>[10x]MAAQNEQRPERIKTTPYLEGDVLSSDSGPLLSVFALQEIMQKVRQVQADYMTATREVDFTVPDVQKILDDIKALAAEQVYKIVKVPSISFRHIVMQSRDRVLRVDTYYEEMSQVGDVITEDEPEKFYSTIIKKVRFIRGKGSFILHDIPTRDHRGMEVAEPEVLGVEFKNVLPVLTAEHRAMIQNALDGSIIENGNVATRDVDVFIGACSEPVYRIYNRLQGYIEAVQLQELRNSIGWLERLGHRKRITYSQEVLTDFRRQDTIWVLALQLPVNPQVVWDVPRSSIANLIMNIATCLPTGEYIAPNPRISSITLTQRITTTGPFAILTGSTPTAQQLNDVRKIYLALMFPGQIILDLKIDPGERMDPAVRMVAGVVGHLLFTAGGRFTNLTQNMARQLDIALNDYLLYMYNTRVQVNYGPTGEPLDFQIGRNQYDCNVFRADFATGTGYNGWATIDVEYREPAPYVHAQRYIRYCGIDSRELINPTTYGIGMTYHCYNEMLRMLVAAGKDSEAAYFRSMLPFHMVRFARINQIINEDLHSVFSLPDDMFNALLPDLIAGAHQNADPVVLDVSWISLWFAFNRSFEPTHRNEMLEVAPLIESVYASELSVMKVDMRHLSLMQRRFPDVLIQARPSHFWKAVLNDSPEAVKAVMNLSHSHNFINIRDMMRWVMLPSLQPSLKLALEEEAWAAANDFEDLMLTDQVYMHRDMLPEPRLDDIERFRQEGFYYTNMLEAPPEIDRVVQYTYEIARLQANMGQFRAALRRIMDDDDWVRFGGVLRTVRVKFYDARPPDDVLQGLPFSYDTNERGGLAYATIKYATETTIFYLIYNVEFSNTPDSLVLINPTYTMTKVFINKRIVERVRVGQILAVLNRRFVAYKGKMRIMDITQSLKMGTKLAAPTV;> MVAITVQGAQLIKRVVERFYPGIAFNINEGACYIYKFSDHIRRIRMKHGTKYRRQAEEIIRNISLRKERLYGIPVLDEVEWKYVFDGQTFQSYAFEVYVNSILPWSELDPEEEFLRNYRVSREMTEVEKFIEFRAKNEMQIYGDIPIKVWCCFINELSAELKHVPLGMQVMADFVNRFDSPFHQGNRDLSNLEDFQVAYTTPLLFEMCCMESILEFNIKMRMREEEISALEFGDMKVDPVGLLREFFILCLPHPKKINNVLRAPYSWFVKMWGVGADPIVVLQSTAGDDRNSKDVFYDKFRTEPNRYKALFRSSFYNESRRMNEEKILEAVKYSQKLGSHDRRLPLFEKMLKTVYTTPFYPHKSSNMILASFLLSIQTITGYGRAWVKNVSTEFDKQLKPNPSNLVQDVSDLTREFFKQAYVEAKERREEIVKPEDLYTSMLRLARNTSSGFSTEIYVKKRFGPRLRDKDLIKINSRIKALVIFTKGHTVFTDEELHKKYNSVELYQTKGSRDVPIKATRTIYSINLSVLVPQLIVTLPLNEYFSRVGGITSPDYKKIGGKVIVGDLEATGSRVMDAADCFRNSADRDIFTIAIDYSEYDTHLTRHNFRTGMLQGIREAMAPYRDLRYEGYTLEQIIDFGYGEGRVANTLWNGKRRLFKTTFDAYIRLDESERDKGSFKVPKGVLPVSSVDVANRIAVDKGFDTLIAATDGSDLALIDTHLSGENSTLIANSMHNMAIGTLMQREVGREQPGVLTFLSEQYVGDDTLFYTKLHTTDTKVFDKVAASIFDTVAKCGHEASPSKTMMTPYSVEKTQTHAKQGCYVPQDRMMIISSERRKDIEDVQG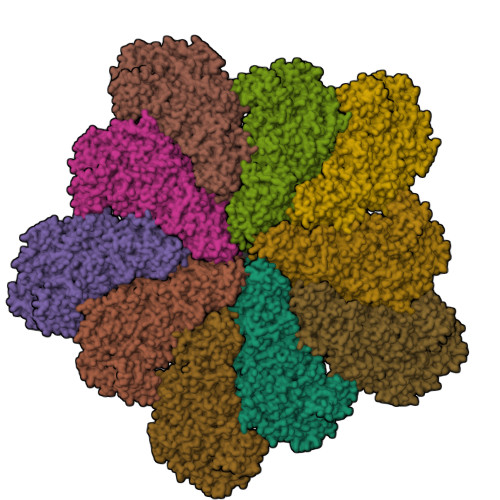YVRSQVQTMITKVSRGFCHDLAQLILMLKTTFIGAWKMKRTIKEDAMYRDRKFDSNDEDGFTLIQIRNPLALYVPIGWNGYGAHPAALNIVMTEEMYVDSIMISKLDEIMAPIRRIVHDIPPCWNETQGDKRGLISATKMSFFSKMARPAVQAALSDPQIINLVEELPLGEFSPGRISRTMMHSALLKESSARTLLSSGYELEYQKALNSWITQVSMRLGEESGVISTSYAKLFDVYFEGELDGAPHMFPDQNLSPQFYIQKMMIGPRVSSRVRNSYVDRIDVILRKDVVMRGFITANTILNVIEKLGTNHSVGDLVTVFTLMNIETRVAEELAEYMTSEKIRFDALKLLKKGIAGDEFTMSLNVATQDFIDTYLAYPYQLTKTEVDAISLYCTQMIMLRAALGLPKKKMKIVVTDDAKKRYKIRLQRFRTHVPKIKVLKKLIDPNRMTVRNLENQFV Argonaute proteins are the central effectors of RNA-guided RNA silencing pathways in eukaryotes, playing crucial roles in gene repression and defense against viruses and transposons. In particular, a deep-branching PIWI protein (HrAgo1) encoded by the genome of the Lokiarchaeon ‘Candidatus Harpocratesius repetitus’ shares a common origin with eukaryotic PIWI proteins. Contrasting known prokaryotic Argonautes that use single-stranded DNA as guides and/or targets, HrAgo1 mediates RNA-guided RNA cleavage, and facilitates gene silencing when expressed in human cells and supplied with miRNA precursors. Thus, this deep-branching archaeal PIWI may have retained an ancestral molecular architecture that preceded the functional and mechanistic divergence of eukaryotic AGOs and PIWIs.

To illuminate the structural basis for RNA-guided RNA cleavage by HrAgo1, we examined HrAgo1 in complex with a 21-nucleotide guide RNA by cryogenic electron microscopy (cryo-EM) and single particle analysis. The resulting reconstruction, determined at a resolution of 3.4 Å, reveals a binary HrAgo1-guide RNA complex. Resembling eAgos and long pAgos, HrAgo1 adopts a bilobed conformation in which one lobe comprises the N-terminal, linker L1, PAZ, and linker L2 domains, connected to the second lobe comprised of the MID and PIWI domains. The first six nucleotides of the guide RNA 5’ end (g1–g6) are ordered in the cryo-EM map. Low-resolution density for four nucleotides at the 3’ end of the guide RNA (g18–g21) is also apparent but uninterpretable, while the remainder of the guide RNA is unstructured. The catalytic tetrad of HrAgo1 comprises residues Asp585, Glu623, Asp655, and His792. In the structure, all four catalytic residues are ordered and in position to mediate divalent cation binding and catalysis, akin to the catalytic site of AGO structures. This implies that HrAgo1 adopts a catalytically active conformation. The negative charge of two phosphates of guide RNA nucleotides 1 and 3, as well as that of the C-terminal carboxyl group of HrAgo1, are neutralized by a Mg2+ ion as is observed in pAgos and PIWIs. In HrAgo1, guide RNA nucleotides g2–g6 are pre-ordered in an A-form-like helical conformation.

> MSKSQNKGRKSNDAPLASPCCPQKKKIDLEMNLFPVKISNLKISIYSWLIFPKIDNYKVQRNILEIALSEEALYEYIIQKNKIYQKKRHPNIKRVVLFQNKEFQIEINHLETVYLLDNPTLQNEIFGSICQTVGFEQIGHNYYYSAERQSSQLTQSTKESLKRIFPAIEIDGGKYYLKQGLTTAIHSTKKNFSIDQGKNAISNVVELEQTSKLIQKKNLLEIIMDLNRKVKDHHKIENLLIGSRFITHYNNRIYTIHGIAWNKDPTSTFQIRSKLHQNLEITFEEYYKKNYQLKISDLHQPLIIYYPMSSQKSATSSGSQDILYFLPEFCHLFGLSNLDADNFRIRQEITRNTQMSPSDRYRKLKTFVENQDILEFFKVWGLDIDSRMISMSGIKLPSLEIQTQTGVFPINFEQSNWLSLLNRSQVIDAPELKKWMILYPKKSMSLQEARKFSNDFQKIAQQMGMVCRPPQLQGVFDMTKFLAILKKNPSQHHINSIQLILTITPNRNKTCYRKIKQLCYRDLGIANQNVVLKNLRDQKRRMPIIRNLVRQIICKVPNFNTKYGGALWKIKNNSIPDKTLIVGIDVWHGRPGIDKSIAGIVFSTDKGLHYTANYTITPRKGLEFIHNLGKIIITQLQNHYNATRQYFENILIFRDGVGNTQYNKILQEEFKSIQQELTNSSIFSEKHPKIAIILVNKRINRRLFHKNKQGQILNPKPGTFIEDQYIKSEFSNYYLVPHFSRFGTTRPIHISVIYNNTKYVNFQFVEIANILCHLNYNWAGTVRIPASVEYAHKVADFIGSNQITSIAPELLQTQFYL9-[2-azido-2-deoxy-5-O-({5-[(3aS,4S,6aR)-2-oxohexahydro-1H-thieno[3,4-d]imidazol-4-yl]pentanoyl}sulfamoyl)-beta-D-arabinofuranosyl]-9H-purin-6-amine 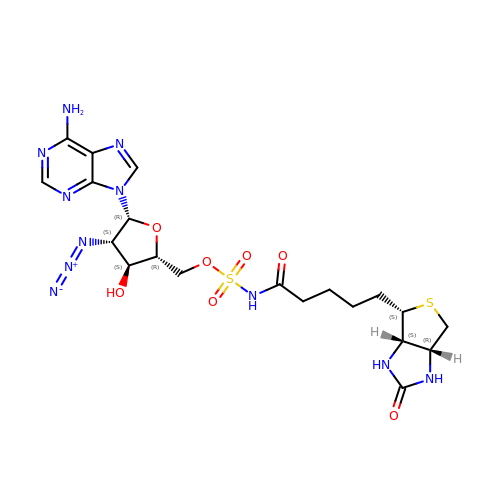| C20 H27 N11 O7 S2 | UYTYJXXHSCNPCG-ROPJLRCXSA-N>[2x]MSRSRPELGDWSSPAELAELQRSQLPRVLAQALRSPFYA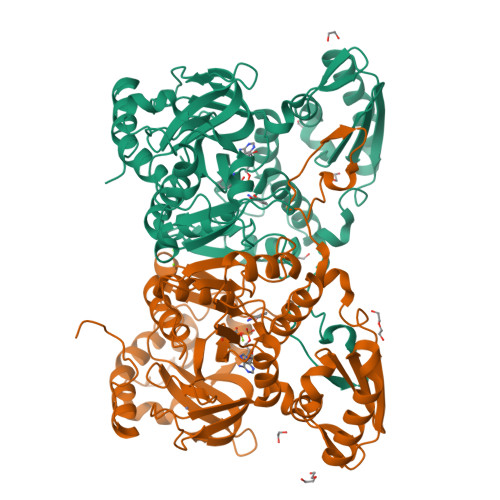ARYRGTTPPRTADDFAGVEVTAKQDLRDQYPFGMLAVGREHLATYHESSGTAGEPTASYYTEEDWTDLAERFARKWTGIHPSDTFLVRTPYGLVITGHLAQAAGRLRGATVVPGDARSLATPLSRMVRVLKTLDVTLTWCNPTEITMLAAAAKAAGLRPDQDFPHLRAMFTAAEPLTEVRRRRLSEIWGGIPVVEEYGSTETGTIAGQCPEGRMHLWADRAIFEVYDPRTGTLSEAGRGQMVVTPLYRDAMPLLRYNLADDVEVSTDPCGCGWLLPTVTVLGRAGTGHRIGPATVTQQRLEELVFSLPAAYEVMFWRAKAHPDVLELEFEAPEPVRQRAVKELGAALDRELGVPHRITGLAPGTLVPAEALTAQRDILKARYLFAEDEDWDKAVMYF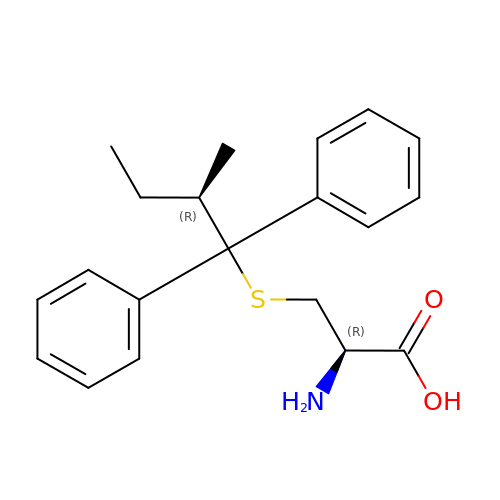(2R)-2-AMINO-3-[(2R)-2-METHYL-1,1-DIPHENYL-BUTYL]SULFANYL-PROPANOIC ACID | C20 H25 N O2 S | AEXWHNCQYTYTMP-QAPCUYQASA-N>QTSVSPSKVILPRGGSVLVTCSTSCDQPKLLGIETPLPKKELLLPGNNRKVYELSNVQEDSQPMCYSNCPDGQSTAKTFLTVYWTPERVELAPLPSWQPVGKNLTLRCQVEGGAPRANLTVVLLRGEKELKREPAVGEPAEVTTTVLVRRDHHGANFSCRTELDLRPQGLELFENTSAPYQLQTFVLPATPPQLVSPRVLEVDTQGTVVCSLDGLFPVSEAQVHLALGDQRLNPTVTYGNDSFSAKASVSVTAEDEGTQRLTCAVILGNQSQETLQTVTIYSFPAPNVILT[2x];>[2x]VDLVFLFDGSMSLQPDEFQKILDFMKDVMKKCSNTSYQFAAVQFSTSYKTEFDFSDYVKRKDPDALLKHVKHMLLLTNTFGAINYVATEVFREELGARPDATKVLIIITDGEATDSGNIDAAKD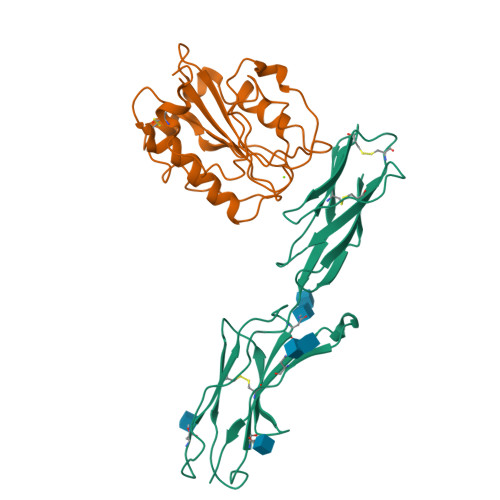IIRYIIGIGKHFQTKESQETLHKFASKPASEFVKILDTFEKLKDLCTELQKKI> MFPYRSLLQTCQPSGSIQGRSGNCNTENGSECCKNGRRYTTYGCSPPVTGSTRAVLTLNSFAEGGDGGGAAACTGKFYDDSKKVVALSTGWYNGGSRCRKHIMIHAGNGNSVSALVVDECDSTVGCDKDHNFE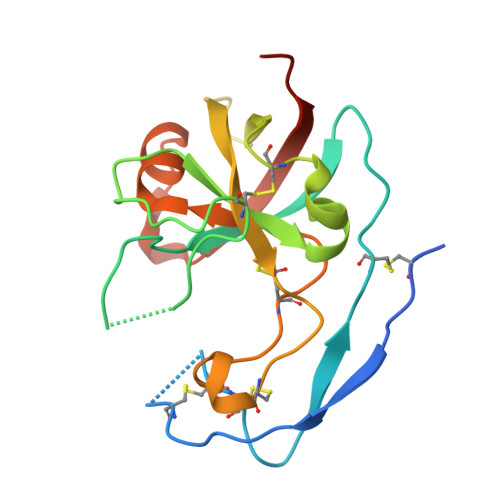PPCRNNIVDGSPAVWDALGLNKDDGQAQITWSDELEHHHHHH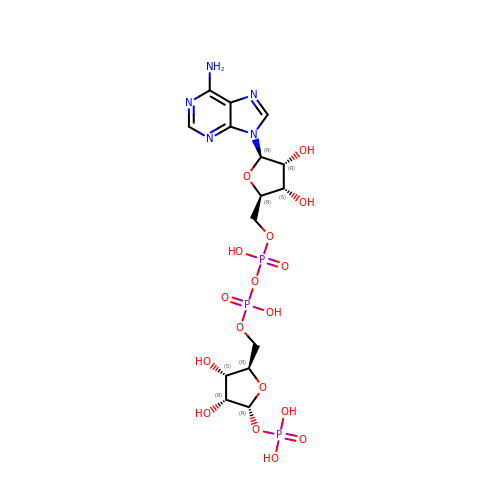[[(2~{R},3~{S},4~{R},5~{R})-5-(6-aminopurin-9-yl)-3,4-bis(oxidanyl)oxolan-2-yl]methoxy-oxidanyl-phosphoryl] [(2~{R},3~{S},4~{R},5~{R})-3,4-bis(oxidanyl)-5-phosphonooxy-oxolan-2-yl]methyl hydrogen phosphate | C15 H24 N5 O17 P3 | CUNFRFHBHMFVPH-KEOHHSTQSA-N>GASGDLYEVERIVDKRKNKKGKWEYLIRWKGYGSTEDTWEPEHHLLHCEEFIDEF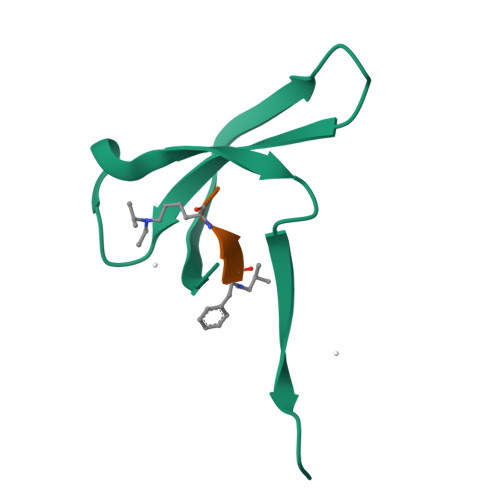NGLHMSK[26x]> SMGFSSELCSPQGHGVLQQMQEAELRLLEGMRKW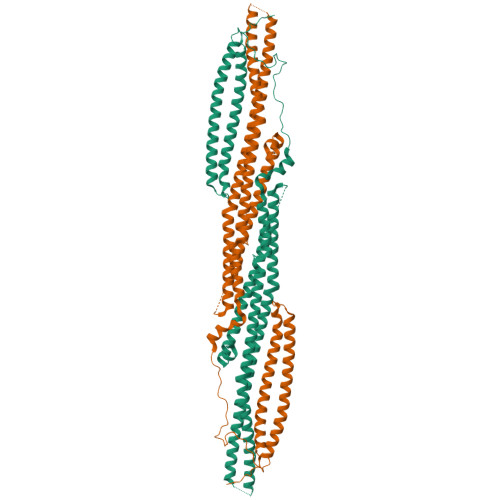MAQRVKSDREYAGLLHHMSLQDSGGQSRAISPDSPISQSWAEITSQTEGLSRLLRQHAEDLNSGPLSKLSLLIRERQQLRKTYSEQWQQLQQELTKTHSQDIEKLKSQYRALARDSAQAKRKYQEASKDKDRDKAKDKYVRSLWKLFAHHNRYVLGVRAAQLHHQHHHQLLLPGLLRSLQDLHEEMACILKEILQEYLEISSLVQDEVVAIHREMAAAAARIQPEAEYQGFLRQYGSAPDVPPCVTFDESLLEEGEPLEPGELQLNELTVESVQHTLTSVTDELAVATEMVFRRQEMVTQLQQELRNEEENTHPRERVQLLGKRQVLQEALQGLQVALCSQAKLQAQQELLQTKLEHLGPGEPPPVLLLQDD>MDENESNQSLMTSSQYPKEAVRKRQNSARNSGASDSSRFSRKSFKLDYRLEEDVTKSKKGKDGRFVNPWPTWKNPSIPNVLRWLIMEKDHSSVPSSKEELDKELPVLKPYFITNPEEAGVREAGLRVTWLGHATVMVEMDELIFLTDPIFSSRASPSQYMGPKRFRRSPCTISELPPIDAVLISHNHYDHLDYNSVIALNERFGNELRWFVPLGLLDWMQKCGCENVIELDWWEENCVPGHDKVTFVFTPSQHWCKRTLMDDNKVLWGSWSVLGPWNRFFFAGDTGYCPAFEEIGKRFGPFDLAAIPIGAYEPRWFMKYQHVDPEEAVRIHTDVQTKKSMAIHWGTFALANEHYLEPPVKLNEALERY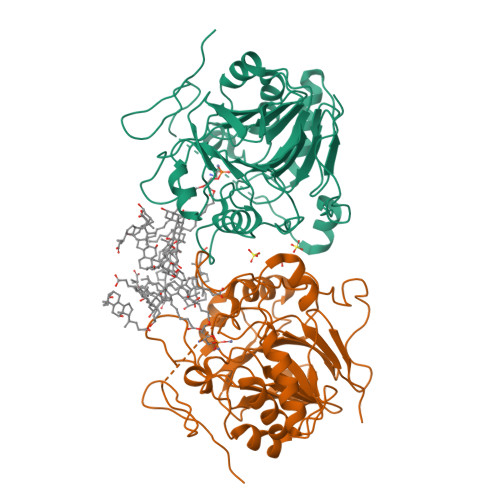GLNAEDFFVLKHGESRYLNNDDENF[2x]> PIFLNVLEAIEPGVVCAGHDNNQPDSFAALLSSLNELGERQLVHVV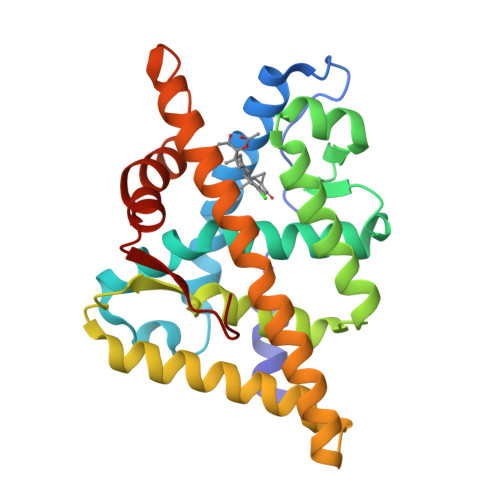KWAKALPGFRNLHVDDQMAVIQYSWMGLMVFAMGWRSFTNVNSRMLYFAPDLVFNEYRMHKSRMYSQCVRMRHLSQEFGWLQITPQEFLCMKALLLFSIIPVDGLKNQKFFDELRMNYIKELDRIIACKRKNPTSCSRRFYQLTKLLDSVQPIARELHQFAFDLLIKSHMVSVDFPEMMAEIISVQVPKILSGKVKPIYFHTQ> MGSSHHHHHHSSGRENLYFQGHMNGLNKG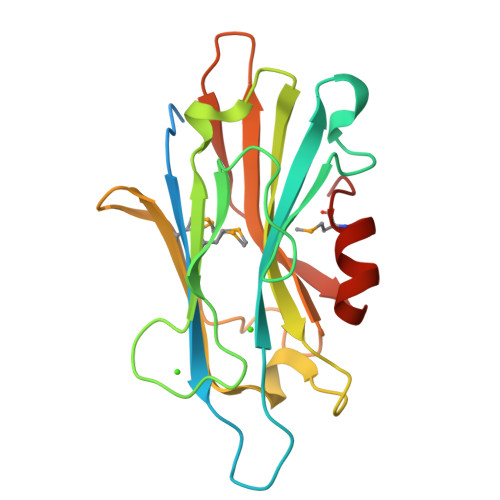IRKVELAVKWDPSPPGDPATDLDIVAATFLAGDAYGKPAYVVHFDSRSPDGTIYLNRDSKDGKGFGWDEVMTLELNRLDSRYARVVVGVVIQQRDAHRTFVGVLNPGLRMREGYTVLAEDDFGGVLGSTAATVGEFVRDDSGEWTFHPGIHGYDSDPATFARVMGGRQDS N,N'-pentane-1,5-diylbis(2,3-dihydroxybenzamide) | C19 H22 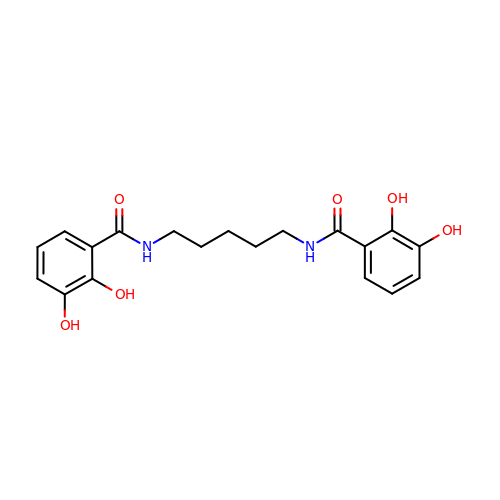N2 O6 | BRWLZTCRFJVZDD-UHFFFAOYSA-N> MKKTLPTKKSNLWFLMACLIITFHKVEAQVPDPNQGLRAEWMRGALGMLWLPERTFNGNIEGIRIDDFLTQIKDIRTVDYVQLPLTSPNIFSPTHVAPHPIIESLWQGDTDANGDPINLVAPRESVDDPLLSWLKALRAAGLRTEIYVNSYNLLARIPEDTQADYPDVSARWMEWCDTNTEAQAFINSQTYHEGNGRRKYMFCYAEFILKEYAQRYGDLIDAWCFDSADNVMEDECGDDPASEDVNDQRIYQAFADACHAGNPNAAIAFNNSVGDREGNPFTSATLFDDYTFGHPFGGAGNMVVPEALYTYNHDLVVFMQTNNGYAFRDDTRTWNDNVVAHFFPKQSTTSWNAGNTPCLTDEQFVEWTSTGIVNGGGITWGTPLVRTNLENAPVLTLQPYALNQFELTDTYLKEFQSPGKPNWSRQYTILPAIYPGQ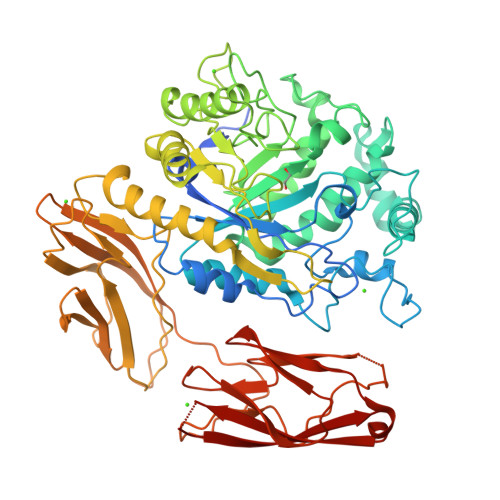PYSHNLVEGVDFWDPEGVGITGLTASGTLPAWLTISQTATGTWTLSGTPPVSEASNYTFELMAQDSDGVTNREVKLEVISHPAGFTNPGDGTPVWFSNPMVLAKATALKDYGSLLKLGVDFYDFEGDVLTITKTSGPDWLVLTQNSDDTWRLSGMPTAADAGENSFTFNVSDGILSSDTEIKITVD> VDLSDEEKDSIYMFASLVEKMKSRPLNEILEDSKLQNLAQRVFASKARLNYALNDKAQKYNTLIEMNGKISEIMNIYDRLLEQQLQSIN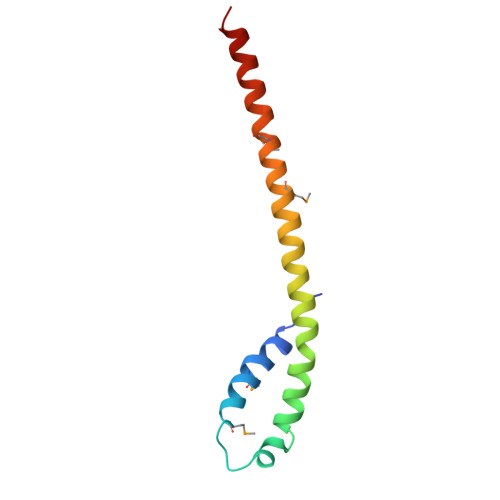LS>HPETLVKVKDAEDQLGARVGYIELDLNSGKILESFRPEERFP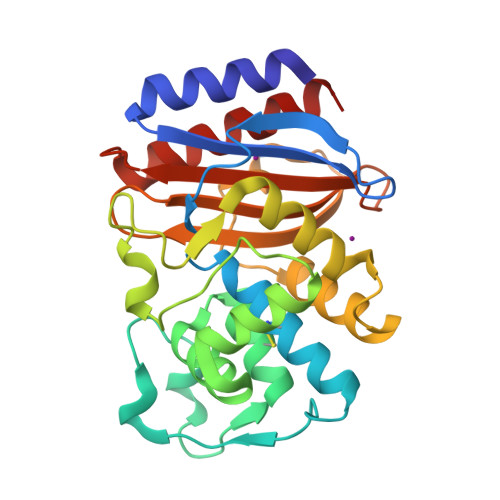MMSTFKVLLCGAVLSRVDAGQEQLGRRIHYSQNDLVEYSPVTEKHLTDGMTVRELCSAAITMSDNTAANLLLTTIGGPKELTAFLHNMGDHVTRLDRWEPELNEAIPNDERDTTTPAAMATTLRKLLTGELLTLASRQQLIDWMEADKVAGPLLRSALPAGWFIADKSGAGERGSRGIIAALGPDGKPSRIVVAYTTGSQATMDERNRQIAEIGASLIKHW[4x]> GAPATVTEQGEDITSKKDRGVLKIVKRVGNGEETPLIGDKVYVHYKGALSNGKKEDSSH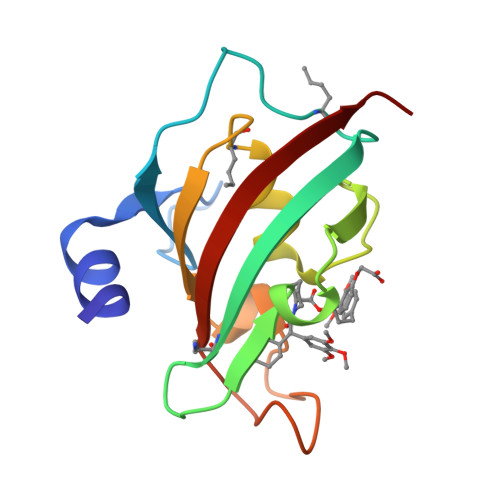DRNEPFVFSLGKGQVIKAWDIGVATLKKGEIAHLLIKPEYAYGSAGSLPKIPSNATLFFEIELLDFKGE>[6x]MLRTMLKSKIHRATVTCA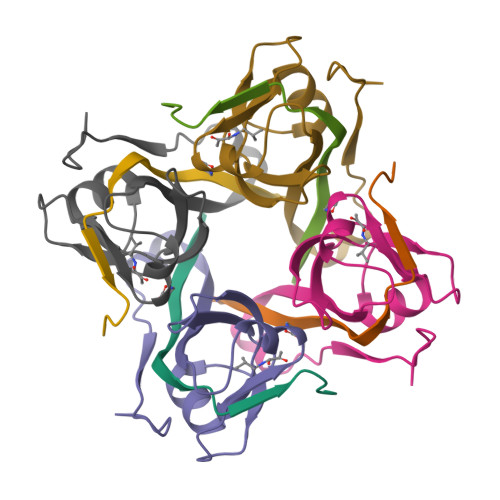DLHYVG;>XVTIDADLMDAADLLEGEQVTIVDIDNGARLVTYAITGERGSGVIGINGAAAHLVHPGDLVILIAYATMDDARARTYQPRIVFVDAYNKPIDMGHDPAFVPENAGELLDPRLGVGLEHHHHHH[6x]> DDDDDDISDDNIKVDPSLKFENPSLRQAYIAL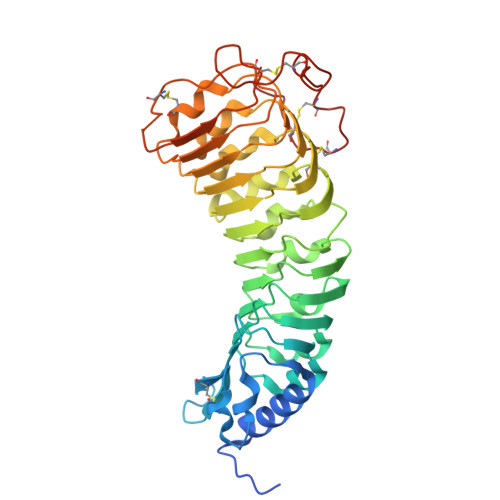QSWKQAIFSDPFNFTANWNGSDVCSYNGIFCAPSPSSPKTRVVAGIDLNHADMAGYLPRELGLLTDLALFHLNSNRFCGEVPLTFKHMKLLFELDLSNNRFVGKFPNVVLSLPSLKFLDLRYNEFEGSIPSKLFDKELDAIFLNHNRFMFGIPENMGNSPVSALVLADNDLGGCIPGSIGLMGKTLNEIILSNDNLTGCLPPQIGNLKNVTVFDISFNRLSGPLPSSIGNMKSLEQLNVANNRFTGVIPSSICQLSNLENFTYSSNFFTGDAPRCVALLGDNVVVNGSMNCIDGKEDQRSSKECSSPASRSVDCSKFGCNNFFSPLENL6-azanyl-2-(2-methoxyethoxy)-9-(pyridin-3-ylmethyl)-7H-purin-8-one | C14 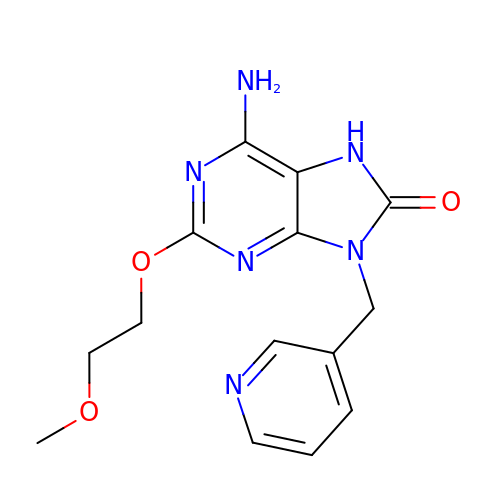H16 N6 O3 | XWTNEKDECZWUJX-UHFFFAOYSA-N>[2x]ATALTNLVAEPFAKLEQDFGGSIGVYAMDTGSGATVSYRAEERFPLCSSFKGFLAAAVLARSQQQAGLLDTPIRYGKNALVPWSPISEKYLTTGMTVAE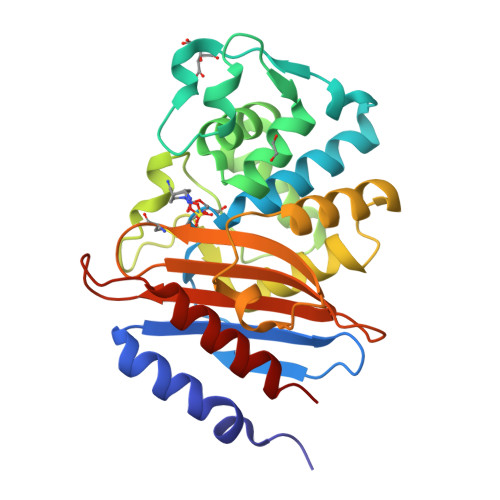LSAAAVQYSDNAAANLLLKELGGPAGLTAFMRSIGDTTFRLDRWELELNSAIPGDARDTSSPRAVTESLQKLTLGSALAAPQRQQFVDWLKGNTTGNHRIRAAVPADWAVGDKTGTCGVYGTANDYAVVWPTGRAPIVLAVYTRAPNKDDKHSEAVIAAAARLALEGLG>[8x]MAAAAGRSLLLLLSSRGGGG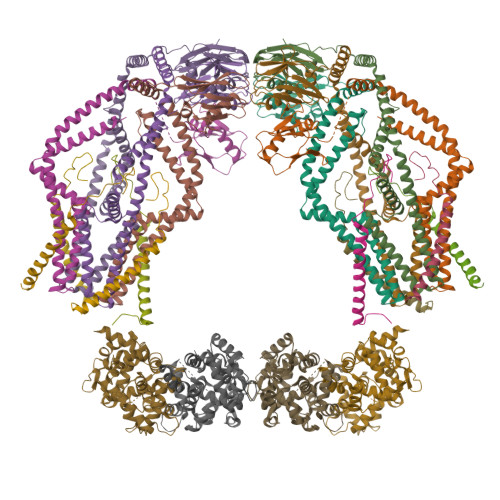GGAGGCGALTAGCFPGLGVSRHRQQQHHRTVHQRIASWQNLGAVYCSTVVPSDDVTVVYQNGLPVISVRLPSRRERCQFTLKPISDSVGVFLRQLQEEDRGIDRVAIYSPDGVRVAASTGIDLLLLDDFKLVINDLTYHVRPPKRDLLSHENAATLNDVKTLVQQLYTTLCIEQHQLNKERELIERLEDLKEQLAPLEKVRIEISRKAEKRTTLVLWGGLAYMATQFGILARLTWWEYSWDIMEPVTYFITYGSAMAMYAYFVMTRQEYVYPEARDRQYLLFFHKGAKKSRFDLEKYNQLKDAIAQAEMDLKRLRDPLQVHLPLRQIGEKD;>MASGAARWLVLAPVRSGALRSGPSLRKDGDVSAAWSGSGRSLVPSRSVIVTRSGAILPKPVKMSFGLLRVFSIVIPFLYVGTLISKNFAALLEEHDIFVPEDDDDDD[8x];>[2x]MFRLNSLSALAELAVGSRWYHGGSQPIQIRRRLMMVAFLGASAVTASTGLLWKRAHAESPPCVDNLKSDIGDKGKNKDEGDVCNHEKKTADLAPHPEEKKKKRSGFRDRKVMEYENRIRAYSTPDKIFRYFATLKVISEPGEAEVFMTPEDFVRSITPNEKQPEHLGLDQYIIKRFDGKKISQEREKFADEGSIFYTLGECGLISFSDYIFLTTVLSTPQRNFEIAFKMFDLNGDGEVDMEEFEQVQSIIRSQTSMGMRHRDRPTTGNTLKSGLCSALTTYFFGADLKGKLTIKNFLEFQRKLQHDVLKLEFERHDPVDGRITERQFGGMLLAYSGVQSKKLTAMQRQLKKHFKEGKGLTFQEVENFFTFLKNINDVDTALSFYHMAGASLDKVTMQQVARTVAKVELSDHVCDVVFALFDCDGNGELSNKEFVSIMKQRLMRGLEKPKDMGFTRLMQAMWKCAQETAWDFALPKQ;>[2x]MAAAAGSCARVAAWGGKLRRGLAVSRQAVRSPGPLAAAVAGAALAGAGAAWHHSRVSVAARDGSFTVSAQKNVEHGIIYIGKPSLRKQRFMQFSSLEHEGEYYMTPRDFLFSVMFEQMERKTSVKKLTKKDIEDTLSGIQTAGCGSTFFRDLGDKGLISYTEYLFLLTILTKPHSGFHVAFKMLDTDGNEMIEKREFFKLQKIISKQDDLMTVKTNETGYQEAIVKEPEINTTLQMRFFGKRGQRKLHYKEFRRFMENLQTEIQEMEFLQFSKGLSFMRKEDFAEWLLFFTNTENKDIYWKNVREKLSAGESISLDEFKSFCHFTTHLEDFAIAMQMFSLAHRPVRLAEFKRAVKVATGQELSNNILDTVFKIFDLDGDECLSHEEFLGVLKNRMHRGLWVPQHQSIQEYWKCVKKESIKGVKEVWKQAGKGLF>[3x]MIISEFDRNNPVLKDQLSDLLRLTWPEEYGDSSAEEVEEMMNPERIAVAAVDQDELVGFIGAIPQYGITGWELHPLVVESSRRKNQIGTRLVNYLEKEVA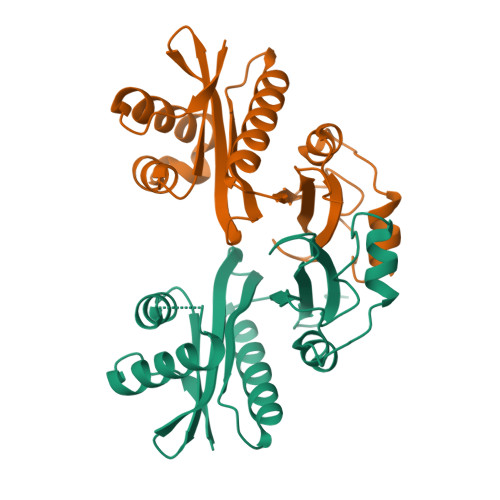SRGGITIYLGTDDLDHGTTLSQTDLYVHTFDKVASIQNLREHPYEFYEKLGYKIVGVLPNANGWDKPDIWMAKTIIPRPDSQ>[2x]GSHMR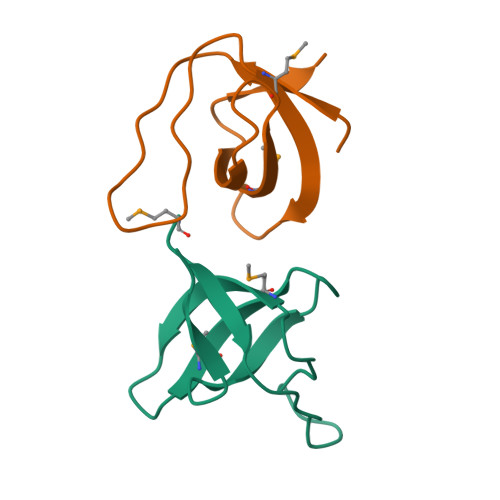RRVRAILPYTKVPDTDEISFLKGDMFIVHNELEDGWMWVTNLRTDEQGLIVEDLVEEVGR>[2x]GSMTIKLLDEFLKKHDLTRYQLSKLTGISQNTLKDQNEKPLNKYTVSILRSLSLI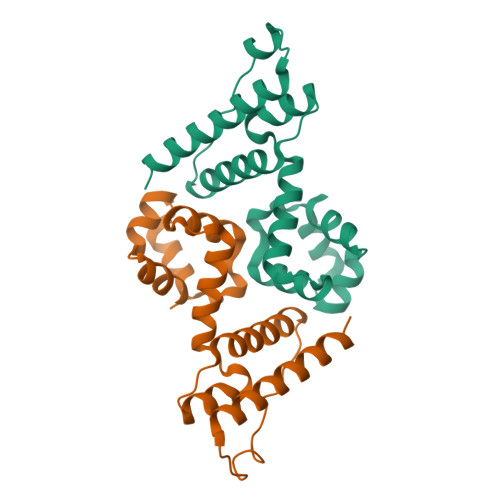SGLSVSDVLFELEDIEKNSDDLAGFKHLLDKYKLSFPAQEFELYCLIKEFESANIEVLPFTFNRFENEEHVNIKKDVCKALENAITVLKEKKNELL The coronavirus surface is studded with spikes that initiate infection by binding to specific cellular receptor(s) leading to membrane fusion and viral entry. Each trimeric spike has a globular crown and a thin stalk anchored to the viral envelope. Each S protomer consists of a N-terminal S1 subunit and a C-terminal S2 subunit. For HCoV-NL63, the S1 subunit is made up of 5 smaller subdomains: 0, A, B, C and D, with domain B acting as the receptor binding domain (RBD) for ACE2.

In the current study we used cryoET and subtomogram averaging to determine the structures of the full-length S ectodomain on virions. Subtomogram averaging analysis of these spikes with imposed C3 symmetry produced an average at 6.9 Å resolution for the crown and lower resolution ~11Å for the upper part of the stalk. To further assess any conformational variability within the S crown, we applied focused classification on both the RBD region and domain 0 region of the three S protomers within each trimeric spike. This analysis confirmed that all three S protomers in a spike are in the pre-fusion, “closed” conformation with all RBDs lying down and no “upward” conformation of domain 0 was detected. Of the 36 on the crown, 29 are predominantly high-mannose glycans (>80%), consistent with reported N-linked glycan profile on HCoV-NL63 S ectodomain produced in Drosophila S2 cells. Spike crowns could be tilted up to 80° relative to the stalk, with a median tilt of 41.6 ± 15°. The averages reveal the significant conformational variability of the trimeric spike through tilting and rotation that are mediated primarily by a large hinge localized to an upper region of the stalk ~100 Å away from the viral envelope. From our simulation results, we determined that most of the bending was localized to the disordered region (residues 1226–1245) separating the two coiled-coil motifs of the stalk. In our stalk model, N-linked glycans at N1242 and N1247 sit between the upper short coiled-coil and lower long coiled-coil and likely contribute to the blob-like density at the bending hinges in spike subtomogram averages. Simulations with the N1242 glycan removed alone bent at comparable angles (Δgly1242 peaks at 20°–25°), which are smaller relative to those with the N1247 glycan removed alone (Δgly1247 peaks at 40°–45°). Removal of N1242 glycan alone or both N1242 and N1247 glycans reduced HCoV-NL63 S mediated infection by ~70% at three different MOIs, in contrast to the negligible effect of removing N1247 glycan alone.

>MKLFLILLVLPLASCFFTCNSNANLSMLQLGVPDNSSTIVTGLLPTHWFCANQSTSVYSANGFFYIDVGNHRSAFALHTGYYDANQYYIYVTNEIGLNASVTLKICKFSRNTTFDFLSNASSSFDCIVNLLFTEQLGAPLGITISGETVRLHLYNVTRTFYVPAAYKLTKLSVKCYFNYSCVFSVVNATVTVNVTTHNGRVVNYTVCDDCNGYTDNIFSVQQDGRIPNGFPFNNWFLLTNGSTLVDGVSRLYQPLRLTCLWPVPGLKSSTGFVYFNATGSDVNCNGYQHNSVVDVMRYNLNFSANSLDNLKSGVIVFKTLQYDVLFYCSNSSSGVLDTTIPFGPSSQPYYCFINSTINTTHVSTFVGILPPTVREIVVARTGQFYINGFKYFDLGFIEAVNFNVTTASATDFWTVAFATFVDVLVNVSATNIQNLLYCDSPFEKLQCEHLQFGLQDGFYSANFLDDNVLPETYVALPIYYQHTDINFTATASFGGSCYVCKPHQVNISLNGNTSVCVRTSHFSIRYIYNRVKSGSPGDSSWHIYLKSGTCPFSFSKLNNFQKFKTICFSTVEVPGSCNFPLEATWHYTSYTIVGALYVTWSEGNSITGVPYPVSGIREFSNLVLNNCTKYNIYDYVGTGIIRSSNQSLAGGITYVSNSGNLLGFKNVSTGNIFIVTPCNQPDQVAVYQQSIIGAMTAVNESRYGLQNLLQLPNFYYVSNGGNNCTTAVMTYSNFGICADGSLIPVRPRNSSDNGISAIITANLSIPSNWTTSVQVEYLQITSTPIVVDCATYVCNGNPRCKNLLKQYTSACKTIEDALRLSAHLETNDVSSMLTFDSNAFSLANVTSFGDYNLSSVLPQRNIRSSRIAGRSALEDLLFSKVVTSGLGTVDVDYKSCTKGLSIADLACAQYYNGIMVLPGVADAERMAMYTGSLIGGMVLGGLTSAAAIPFSLALQARLNYVALQTDVLQENQKILAASFNKAINNIVASFSSVNDAITQTAEAIHTVTIALNKIQDVVNQQGSALNHLTSQLRHNFQAISNSIQAIYDRLDSIQADQQVDRLITGRLAALNAFVSQVLNKYTEVRGSRRLAQQKINECVKSQSNRYGFCGNGTHIFSIVNSAPDGLLFLHTVLLPTDYKNVKAWSGICVDGIYGYVLRQPNLVLYSDNGVFRVTSRVMFQPRLPVLSDFVQIYNCNVTFVNISRVELHTVIPDYVDVNKTLQEFAQNLPKYVKPNFDLTPFNLTYLNLSSELKQLEAKTASLFQTTVELQGLIDQINSTYVDLKLLNRFENYIKWPWWVWLIISVVFVVLLSLLVFCCLSTGCCGCCNCLTSSMRGCCDCGSTKLPYYEFEKVHVQ[3x]> MSVGLIAPLASPIQESRANTNIENIGDGAEVIKRTEDVSSKKWGVTQNVQFDFVKDKKYNKDALIVKMQGFINSRTSFSDVKGSGYELTKRMIWPFQYNIGLTTKDPNVSLINYLPKNKIETTDVGQTLGYNIGGNFQSAPSIGGNGSFNYSKTISYTQKSYVSEVDKQNSKSVKWGVKANEFVTPDGKKSAHDRYLFVQSPNGPTGSAREYFAPDNQLPPLVQSGFNPSFITTLSHEKGSSDTSEFEISYGRNLDITYATLFPRTGIYAERKHNAFVNRNFVVRYEVNWKTHEIKVK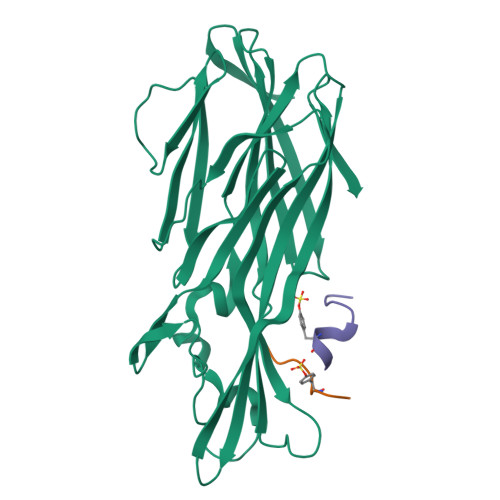GHNKHHHHHH;>XDSFPDGDYGANLE[2x]>[2x]SRKTYTLTDYLKNTYRLKLYSLRWISDHEYLYKQENNILVFNAEYGNSSVFLENSTFDEFGHSINDYSISPDGQFILLEYNYVKQWRHSYTASYDIYDLNKRQLITEERIPNNTQWVTWSPVGHKLAYVWNNDIYVKIEPNLPSYRITWTGKEDIIYNGITDWVYEEEVFSAYSALWWSPNGTFLAYAQFNDTEVPLIEYSFYSDESLQYPKTVRVPYPKAGAVNPTVKFFVVNTDSLSSVTNATSIQITAPASMLIGDHYLCDVTWATQERISLQWLRRIQNYSVMDICDYDESSGRWNCLVARQHIEMSTTGWVGRFRPSEPH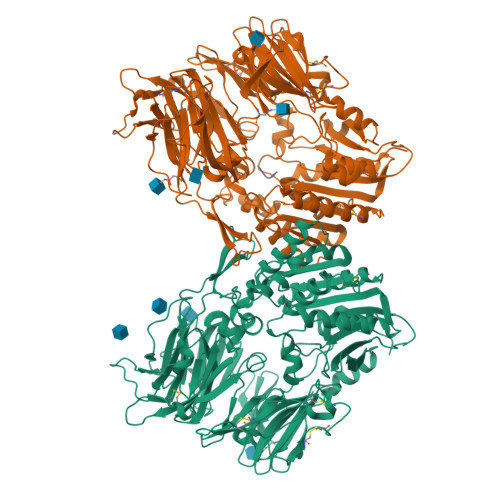FTLDGNSFYKIISNEEGYRHICYFQIDKKDCTFITKGTWEVIGIEALTSDYLYYISNEYKGMPGGRNLYKIQLSDYTKVTCLSCELNPERCQYYSVSFSKEAKYYQLRCSGPGLPLYTLHSSVNDKGLRVLEDNSALDKMLQNVQMPSKKLDFIILNETKFWYQMILPPHFDKSKKYPLLLDVYAGPCSQKADTVFRLNWATYLASTENIIVASFDGRGSGYQGDKIMHAINRRLGTFEVEDQIEAARQFSKMGFVDNKRIAIWGWSYGGYVTSMVLGSGSGVFKCGIAVAPVSRWEYYDSVYTERYMGLPTPEDNLDHYRNSTVMSRAENFKQVEYLLIHGTADDNVHFQQSAQISKALVDVGVDFQAMWYTDEDHGIASSTAHQHIYTHMSHFIKQCFSLP;> IPI> MENVTESKELERLKRIDRMKTEFIANISHELRTPLTAIKAYAETIYNSLGELDLSTLKEFLEVIIDQSNHLENLLNELLDFSRLERKSLQINREKVDLCDLVESAVNAIKEFASSHNVNVLFESNVPCPVEAYIDPTRIRQVLLNLLNNGVKYSKKDAPDKYVKVILDEKDGGVLIIVEDNG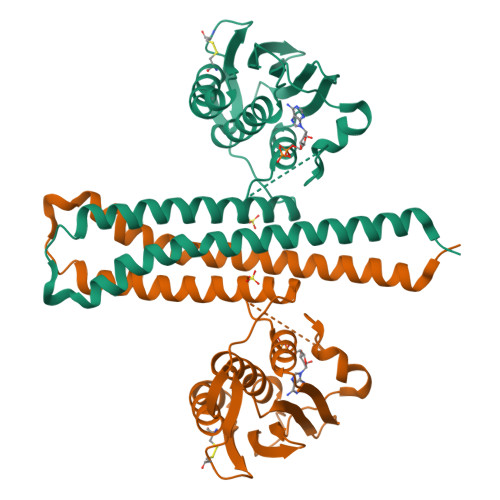IGIPDHAKDRIFEQFYRVDSSLTYEVPGTGLGLAITKEIVELHGGRIWVESEVGKGSRFFVWIPKDRAGEDNRQDN>[9x]SSDTTPCCFAYIARPLPRAHIKEYFYTSGKCSNPAVVFVTRKNRQVCANPEKKWVR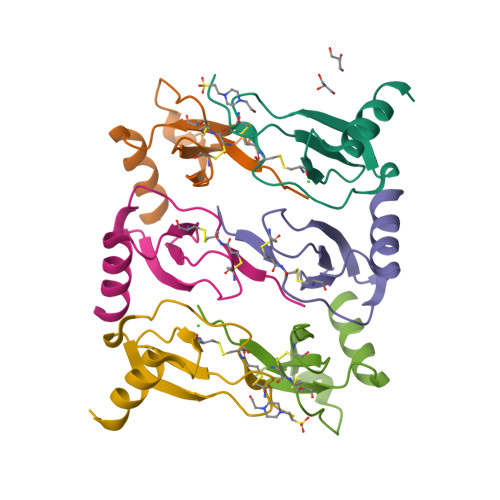EYINSLEMS>[4x]GSGAPPTDLQKMVMGNTKPVELILDGKTVAICCATGVFGTAYLVPRHLFAEKYDKIMLDGRAMTDSDYRVFEFEIKVKGQDM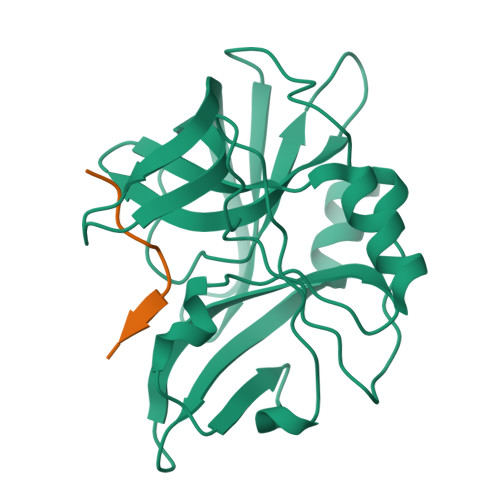LSDAALMVLHRGNKVRDITKHFRDTARMKKGTPVVGVVNNADVGRLIFSGEALTYKDIVVLMDGDTMPGLFAYKAATRAGYAGGAVLAKDGADTFIVGTHSAGGNGVGYCSCVSRSMLQKMKAHVDPEPHHE;>[4x]XAPAKELLNFD[[(2~{R},3~{R},4~{R},5~{R})-5-(6-aminopurin-9-yl)-4-oxidanyl-3-phosphonooxy-oxolan-2-yl]methoxy-oxidanyl-phosphoryl] 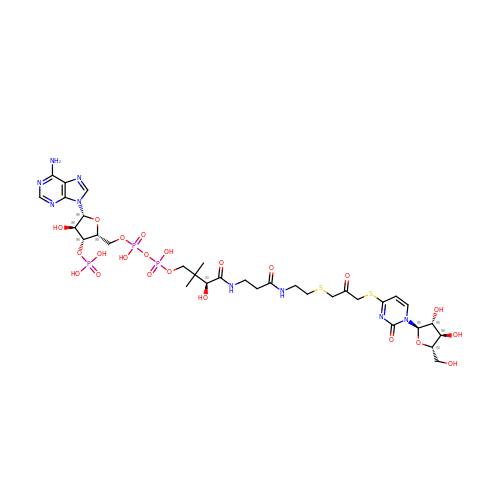[(3~{S})-4-[[3-[2-[3-[1-[(2~{R},3~{R},4~{R},5~{S})-5-(hydroxymethyl)-3,4-bis(oxidanyl)oxolan-2-yl]-2-oxidanylidene-pyrimidin-4-yl]sulfanyl-2-oxidanylidene-propyl]sulfanylethylamino]-3-oxidanylidene-propyl]amino]-2,2-dimethyl-3-oxidanyl-4-oxidanylidene-butyl] hydrogen phosphate | C33 H50 N9 O22 P3 S2 | XSHNUOJAICKWRY-KAESTEPRSA-N>SRCTHLENRDFVTGTQGTTRVTLVLELGGCVTITAEGKPSMDVWLDAIYQENPAKTREYCLHAKLSDTKVAARCPTMGPATLAEEHQGGTVCKRDQSDRGWGNHCGLFGKGSIVACVKAACEAKKKATGHVYDANKIVYTVKVEPHTGDYVAANETHSGRKTASFTVSSEKTILTMGEYGDVSLLCRVASGVDLAQTVILELDKTVEHLPTAWQVHRDWFNDLALPWKHEGAQNWNNAERLVEFGAPHAVKMDVYNLGDQTGVLLKALAGVPVAHIEGTKYHLKSGHVTCEVGLEKLKMKGLTYTMCDKTKFTWKRAPTDSGHDTVVMEVTFSGTKPCRIPVRAVAHGSPDV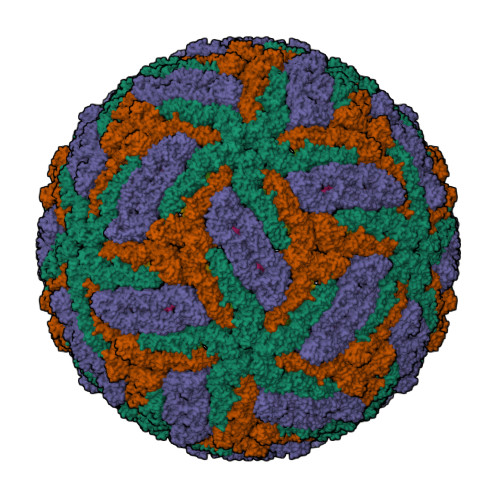NVAMLITPNPTIENNGGGFIEMQLPPGDNIIYVGELSHQWFQKGSSIGRVFQKTKKGIERLTVIGEHAWDFGSAGGFLSSIGKAVHTVLGGAFNSIFGGVGFLPKLLLGVALAWLGLNMRNPTMSMSFLLAGGLVLAMTLGVGA[3x];>[3x]SVLIPSHAQGELTGRGHKWLEGDSLRTHLTRVEGWVWKNKLLALAMVTVVWLTLESVVTRVAVLVVLLCLAPVYA>GSHMEQLKHCNGILKELLSKKHAAYAWPFYKPVDASALGLHDYHDIIKHPMDLSTVKRKMENRDYRDAQEFAADVRLM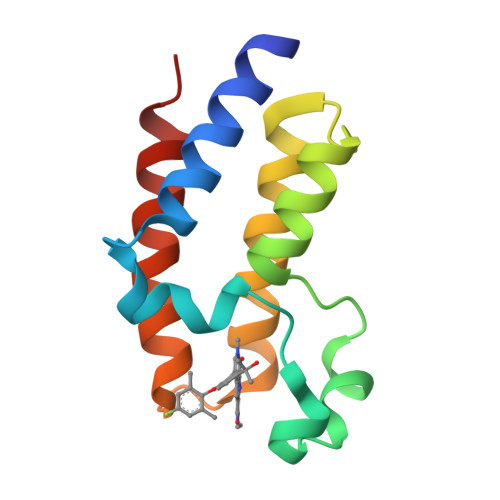FSNCYKYNPPDHDVVAMARKLQDVFEFRYAKMPD[6x]> MHHHHHHENLYFQGTKDLNTLVSELPEIYQTIFGHPEWDGDAARDCNQRLDLITEQYDNLSRALGRPLNVLDLGCAQGFFSLSLASKGATIVGIDFQQENINVCRALAEENPDFAAEFRVGRIEEVIAALEEGEFDLAIGLSVFHHIVHLHGIDEVKRLLSRLADVTQAVILELAVKEEPFYWGVSQPDDPRELIEQCAFYRLIGEFDTH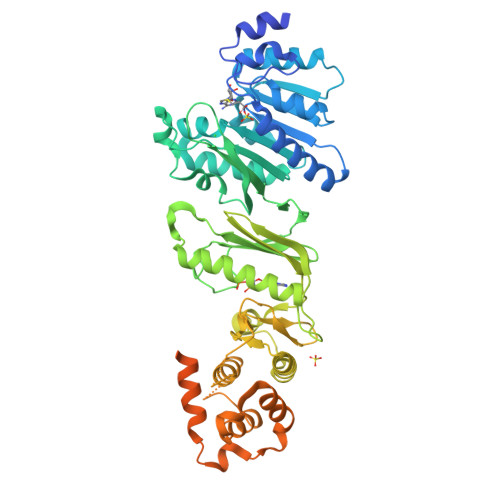LSPVPRPMYLVSNHRVLINDFNQPFQHWQNQPYAGAGLAHKRSRRYFFGEDYVCKFFYYDMPHGILTAEESQRNKYELHNEIKFLTQPPAGFDAPAVLAHGENAQSGWLVMEKLPGRLLSDMLAAGEEIDREKILGSLLRSLAALEKQGFWHDDVRPWNVMVDARQHARLIDFGSIVTTPQDCSWPTNLVQSFFVFVNELFAENKSWNGFWRSAPVHPFNLPQPWSNWLYAVWQEPVERWNFVLLLALFEKKAKLPSAEQQRGATEQWIIAQETVLLELQSRVRNESAGSEALRGQIHTLEQQMAQLQSAQDAFVEKAQQQVEVSHELTWLGENMEQLAALLQTAQAHAQADVQPELPP> ACQCPDAISGWTHTDYQCHGLENKMYRHVYAICMNGTQVYCRT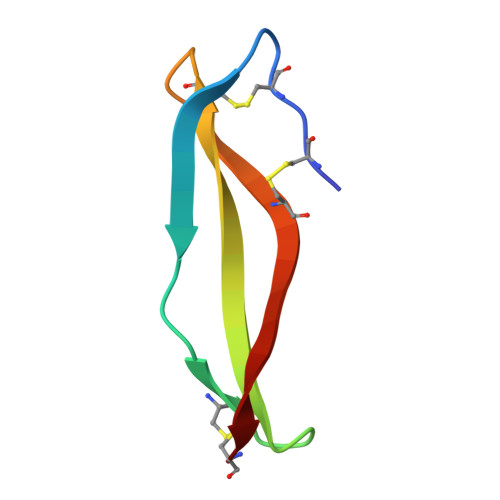EWGSSC>GPDSASRISPGQINQVRPKLPLLKILHAAGAQGEMFTVKEVMHYLGQYIMVKQLYDQQEQHMVYCGGDLLGELLGRQSF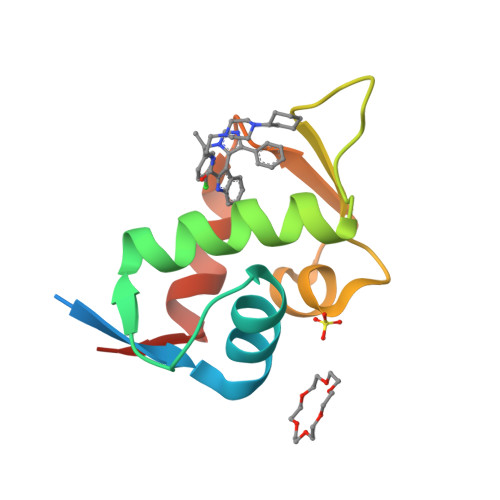SVKDPSPLYDMLRKNLVTLAT[4x]Ssr4 is a yeast protein from Schizosaccharomyces pombe and is an essential part of the chromatin-remodelling [SWI/SNF and RSC (remodelling the structure of chromatin)] complexes found in S. pombe. These complexes (or their homologues) regulate gene expression in eukaryotic organisms, affecting a large number of genes both positively and negatively. The chromatin structure is altered by modifying the DNA–histone contacts, thus opening up or closing down sections of DNA to specific transcription factors that regulate the transcription of genes. The structure of the N-terminal domain is an antiparallel β-sheet of seven strands with α-helices on one side and random coil on the other.

The Ssr4 sequence has little homology to other sequences in the Protein Data Bank, so the structure was solved using an iodine derivative with SAD phasing. As there were no homologous structures in the PDB which might serve as a molecular-replacement model for this protein structure, we attempted to use several different methods for de novo phasing: xenon, bromine and iodine soaks and native sulfur SAD phasing. The Ssr4 structure was solved using a crystal that had been soaked with iodine and which showed two major peaks for I atoms in the electron density (about 40σ and 30σ above the background), with three more peaks (12σ, 11σ and 5.5σ) that corresponded to either low-occupancy I or Cl atoms (some of these peaks are also seen in non-iodine-soaked structures). Auto-Rickshaw was used to find the iodines, phase the data and build the initial structure via Buccaneer. Although the sulfur, bromine and iodine data sets all showed some anomalous signal in the scaled statistics, only the iodine data set had sufficient signal to solve the structure. Density was seen for residues extending from the N-terminal tag to residue 179/180 of the Ssr4 protein in all three structures. The N-terminal tag used for purification forms a helix from residues −9 to −2 and there is a break in the density in two of the three structures where the residues Ser1 and Ala2 should reside (Ser1 is the last residue of the tag and Ala2 is the first residue of native Ssr4). These two residues were modelled into one of the models as there is some weak density in the iodine-phased data, with a break at Gly0. We have crystallized and solved the structure of the N-terminal domain (up to residue ∼180 of 395) of Ssr4 using an iodine derivative.

> MGHHHHHHGTENLYFQGSAATMAAQSLLSIPVEYRSQVWCRANLPYPPAPQLPIPAVVDILTKASQALPQISFSWTLIDQPPDGSLFLVWQAPTLPSPPDGMHFMSNERFFNMDVAGKVLEIHEAKHGFYPLSETRTMHVRCRYRLLGVGFDNFWLVHYFQGSETDSIPANISVAKPPHLRRYPLPDVKTSPFLLQE> AGGGTTAGGGTTAGGGTTAGGG

Quadruplex DNA and RNA are higher-order arrangements formed by nucleic acid sequences containing tandem repeats of short G-tracts. Quadruplex structures comprise a core of G-quartets, connected by variable-sequence nucleotide loops. A quartet itself comprises four in-plane guanine bases bound by Hoogsteen G:G base pairing, and held together by the sugar-phosphate backbone. We report here on an analysis of the hydration arrangements around selected folded quadruplex DNAs, which has revealed several prominent features that re-occur in related structures.

In parallel quadruplexes, typified by the human telomeric quadruplex crystal structures, all G-bearing strands are oriented in the same direction and all grooves are of medium width. Three propeller T–T–A loops extend across three of the grooves. Because of the geometry of Hoogsteen base pairs in the G-quartets, the only non-carbon atoms at the floor of the grooves accessible to hydrogen bonding are N2/N3. Those N2/N3 atoms are always observed to be on the same side of the medium groove, for example the left-hand side in Figure 2A. The guanosines adopt an anti glycosidic conformation and the O4′ of the deoxyribose sugar is oriented into the groove on the N2/N3 side, and outwards on the C8 side. The N2/N3 + O4’ → phosphate water bridges pull the sides of the grooves together. And because the guanosines with a C8 atom in the floor of groove have their N2/N3 side forming the floor of the adjacent groove, these bridges continue across all the grooves, forming in effect a water ribbon wrapping around the quadruplex and further stabilizing the overall structure. The conformations of T–T–A loops in parallel quadruplexes have been found to be maintained by the water networks within and adjacent to the loops. Most phosphates of loop nucleotides point inward and are connected by the dense water clusters (i.e. phosphate → phosphate water contacts). The groove defined by G20–G2 is the only groove not obstructed by the propeller loop, therefore, the phosphate → phosphate water connectivity is not observed here.> MSTVATYSYTHSVTYVTDNILKSLKDIILLSGLDPEHFADRWESNTRAIKTW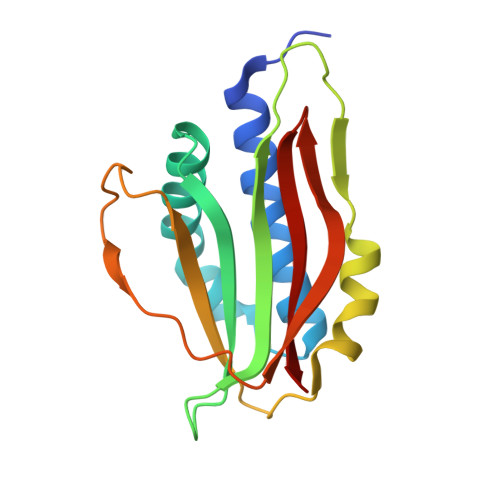LGTGDLRKVILEIYNPATDKLVTRWDIDIVYGWSDGDGSFWTDTEQLKYAIKKAGLLPSQAKYKLMLDTKPGRPDVEGWSKGSYRSTDGMVKQSLGSTVEHSGLAGQAGYWRQR>[2x]MSLAIKLIAIDMDGTLLLPDHTISPAVKNAIAAARARGVNVVLTTGRPYA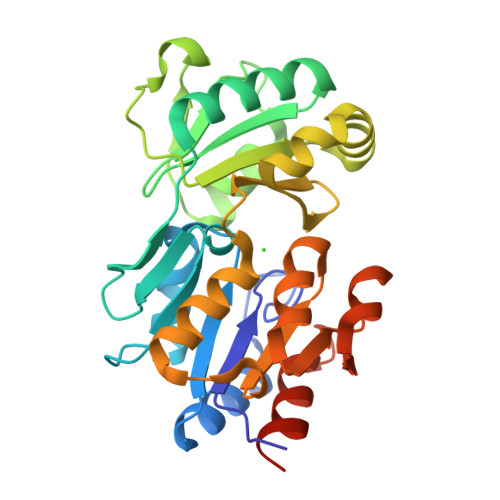GVHNYLKELHMEQPGDYCITYNGALVQKAADGSTVAQTALSYDDYRFLEKLSREVGSHFHALDRTTLYTANRDISYYTVHESFVATIPLVFCEAEKMDPNTQFLKVMMIDEPAILDQAIARIPQEVKEKYTVLKSAPYFLEILDKRVNKGTGVKSLADVLGIKPEEIMAIGDQENDIAMIEYAGVGVAVDNAIPSVKEVANFVTKSNLEDGVAFAIEKYVLNEGGSHHHHHH>[2x]SNAMASQSRLTFVNLPVADVAASQAFFGTLGFEFNPKFTDESCACMVVSEQAFVMLIDRARFADFTSKPIADATATTEAIVCVSAID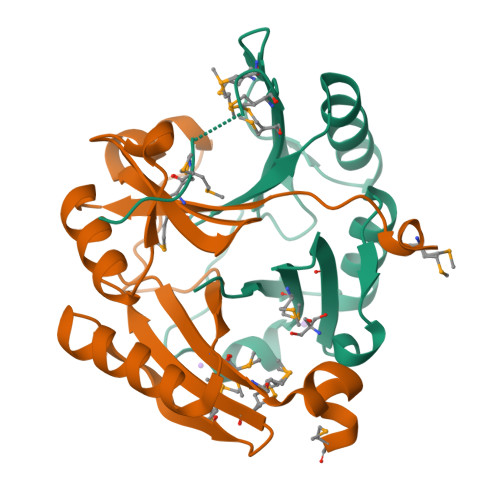RDDVDRFADTALGAGGTVARDPMDYGFMYGRSFHDLDGHLWEVMWMSAEAVEQGPADMAQPV[(3~{S},4~{R})-4-(6-oxidanylidene-1~{H}-purin-9-yl)pyrrolidin-3-yl]oxymethylphosphonic 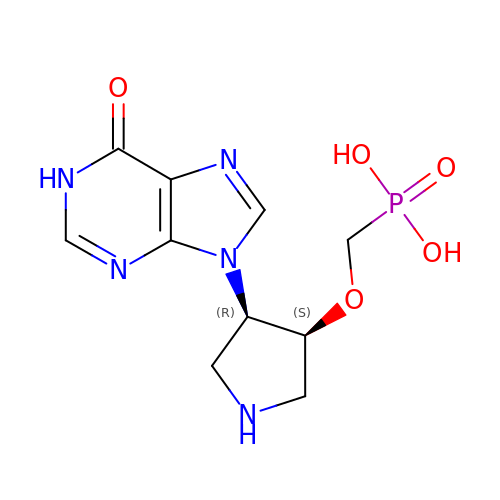acid | C10 H14 N5 O5 P | YFBRPISOXMPUHB-RQJHMYQMSA-N>GSHMASMLLDTFQGYNCYSSALGEYAKQKNIDQVENIILSQWSFFFDEEQFYKNQWYTGAADGPVDVVLN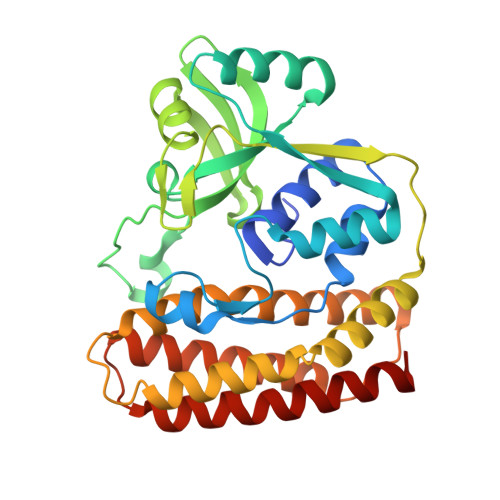EDLRNFANIEVLEHISSESQAIDEGRKVLEKHGLQIVLMDFYYMNSFNWKSLSRFNVTREHDPAFAVLTQINENSVHIIDPYYHHEENMSMEDFIKSRNSMTKQGKISFNSYEIFSNGTKKSNIKELLYYRFNRYLQEKMFGKITQFGQVVKKQLDNKDRKWAFTGYNCLNSVVYQHQNLINLQKKFSLEMPPNLQELLDNWALIRKKLFEYYSRGSYNTEEISNLICKVASSEEQFAQEVLKVL[2x]>[2x]MNSNLPAENLTIAVNMTKTLPTAVTHGFNSTNDPPSMSITRLFPALLECFGIVLCGYIAGRANVITSTQAKGLGNFVSRFALPALLFKNMVVLNFSNVDWSFLYSILIAKASVFFIVCVLTLLVASPDSRFSKAGLFPIFATQSNDFALGYPIVEALYQTTYPEYLQYIYLVAPISLMMLNPIGFIFCEIQKWKDTQNASQ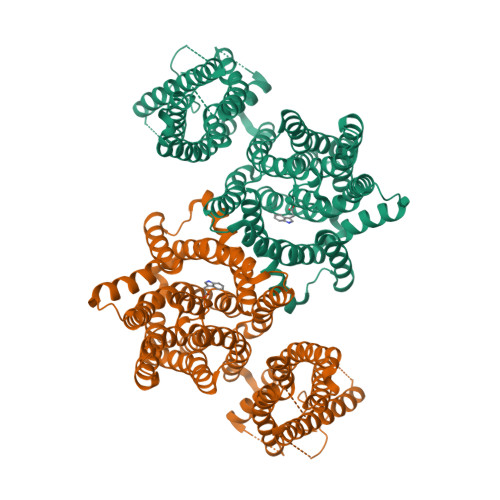NKIKIVGLGLLRVLQNPIVFMVFIGIAFNFILDRKVPVYVENFLDGLGNSFSGSALFYLGLTMVGKIKRLKKSAFVVLILLITAKLLVLPLLCREMVELLDKGDSVVNHTSLSNYAFLYGVFPVAPGVAIFATQFNMEVEIITSGMVISTFVSAPIMYVSAWLLTFPTMDPKPLAYAIQNVSFDISIVSLISLIWSLAILLLSKKYKQLPHMLTTNLLIAQSIVCAGMMIWNFVKEKNFVGQILVFVLLYSSLYSTYLWTGLLAISLFLLKKRERVQIPVGIIIISGWGIPALLVGVLLITGKHNGDSIDSAFFYGKEQMITTAVTLFCSILIAGISLMCMNQTAQAGSYEGFDQSQSHKVVEPGNTAFEESPAPVNEPELFTSSIPETSCCSCSMGNGELHCPSIEPIANTSTSEPVIPSFEKNNHCVSRCNSQSCILAQEEEQYLQSGDQQLTRHVLLCLLLIIGLFANLSSCLWWLFNQEPGRLYVELQFFCAVFNFGQGFISFGIFGLDKHLIILPFKRRLEFLWNNKDTAENRDSPVSEEIKMTCQQFIHYHRDLCIRNIVKERRCGAKTSAGTFCGCDLVSWLIEVGLASDRGEAVIYGDRLVQGGVIQHITNEYEFRDEYLFYRFLQKSPEQSPPAINANTLQQERYKEIEHSSPPSHSPKTGSGSDYKDDDDKDYKDDDDK> MKEKKKEIEKLLARPDLTPEQMKNYGMEYAKIEEIENITNRIKETQEFIELLREEGE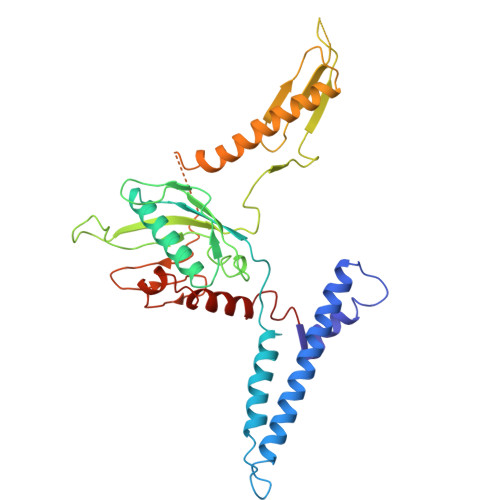NELEIEKYEKELDQLYQELLFLLSPEASDKAIVEIRPGTGGEEAALFARDLFRMYTRYAERKGWNLEVAEIHETDLGGIREVVFFVKGKNAYGILKYESGVHRVQRVPVTESGGRIHTSTATVAVLPEIEEKDIEIRPEDLKIETFRASGHGGQYVNKTESAVRITHLPTGIVVSCQNERSQYQNKQTALRILRARLYQLQKEQKEREISQKRKSQIGTGERSEKIRTYNFPQNRVTDHRINYTSYRLQEILDGDLDEIISKLIEHDIENNLEEVL> GSDELYRQSLE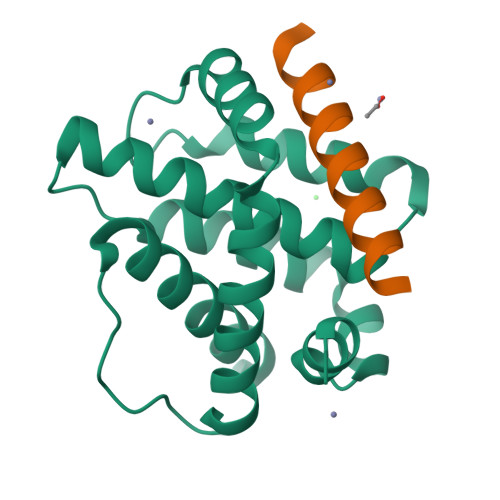IISRYLREQATGAKDTKPMGRSGATSRKALETLRRVGDGVQRNHETAFQGMLRKLDIKNEDDVKSLSRVMIHVFSDGVTNWGRIVTLISFGAFVAKHLKTINQESCIEPLAESITDVLVRTKRDWLVKQRGWDGFVEFFHVEDLEGG;> RPEIWAAQELRRIGDEFNAYYR>[4x]MNQT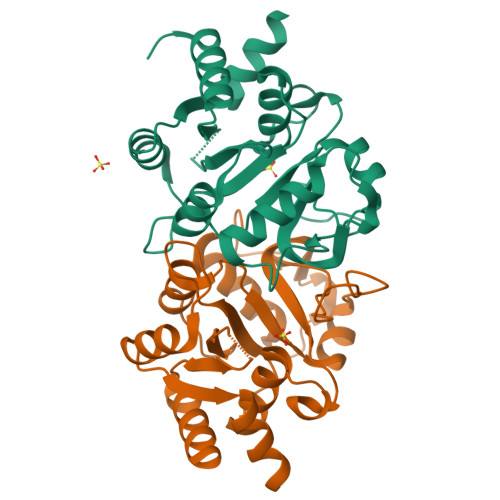LLSSFGTPFERVELALDALREGRGVMVLDDEDRENEGDMIFPAETMTVEQMALTIRHGSGIVCLCITEDRRKQLDLPMMVENNTSAYGTGFTVTIEAAEGVTTGVSAADRVTTVRAAIKDGAKPSDLNRPGHVFPLRAQAGGVLTRGGHTEATIDLMTLAGFKPAGVLCELTNDDGTMARAPECIAFAGQHNMAVVTIEDLVAYRQAHERKAS>SNAMETFLFTSESVNEGHPDKLCDQISDAVLDACLEQDPDSKVACETCTKTNMVMVFGEITTKATIDYEKIVRDTCRSIGFISDDVGLDADKCKVLVNIEQQSPDIAQGVHGHFTKRPEDIGAGDQGHMFGYATDETPELMPLSHVLATKIGARLTEVRKNGTCRWLRPDGKTQVTVEYYNDNGAMVPVRVHTVLISTQHDETVTNDEIARDLKEHVIKPIIPEKYLDDKTIFHLNPSGRFVIGGPHGDAGLTGRKIIIDTYGGWG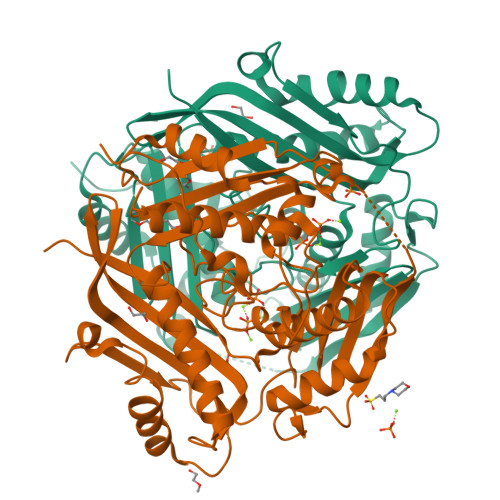AHGGGAFSGKDPTKVDRSGAYIVRQAAKSVVANGMARRALVQVSYAIGVPEPLSVFVDTYGTGLIPDKEILKIVKETFDFRPGMMTINLDLKRGGNGRFQKTAAYGHFGRDDPDFTWEVVKPLKWDKPQLNNIGSG[2x]> MGRLVGLELSNFKSYRGVTKVGFGESNFTSIIGPNGSGKSNMMDAISFVLGVRSNHLRSNILKDLIYRGVLNDENSDDYDNEGAASSNPQSAYVKAFYQKGNKLVE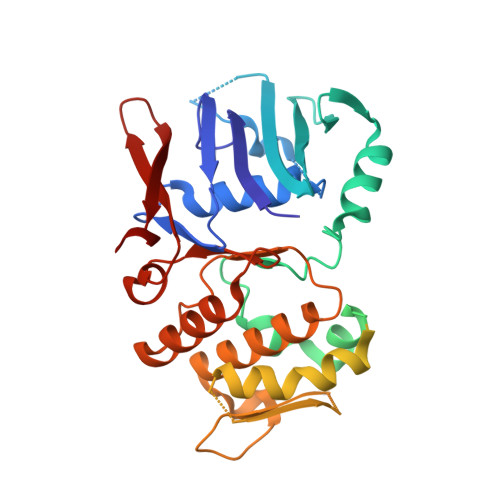LMRIISRNGDTSYKIDGKTVSYKDYSIFLENENILIKAKNFLVFQGDVEQIAAQSPVELSRMFEEVSGSIQYKKEYEELKEKIEKLSKSATESIKNRRRIHGELKTYKSPGLEVLFQGPRGSRYDEAEGRFEVINNETEQLKAEEKKILNQFLKIKKKRKELFEKTFDYVSDHLDAIYRELTKNPNSNVELAGGNASLTIEDEDEPFNAGIKYHATPPLKRFKDMEYLSGGEKTVAALALLFAINSYQPSPFFVLDEVDAALDITNVQRIAAYIRRHRNPDLQFIVISLKNTMFEKSDALVGVYRQQQENSSKIITLDLSNYAE>MQRLSPGEFKTLISKERKSHFITPFALVYKTFCDLGYDQKNSDYFLNNPSEYIIAMRKNCWKEFEPFEKEFTTRMLSYLIDEERIKDMSPYDAIRDFTMEYPTHIYDLALSNTQSRRSRAGKEFESILELLMMGAGIPVD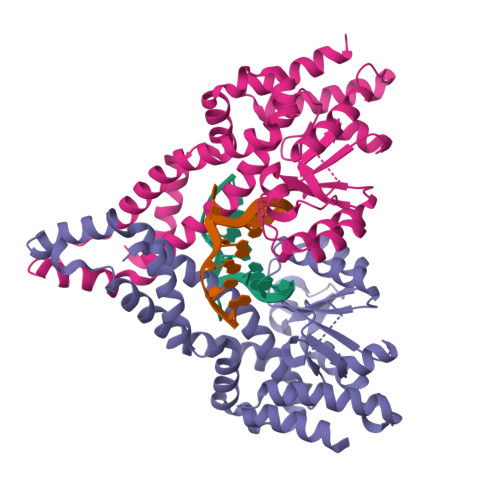VQGAIGKSFFQKNQIGKLVDLVMPGVVQYTSNKRNTMLISAKTTLRERWQEVPEEVNRTGIREMYLATLDDSFSEETINILYEANVVVVTTVENKNFKYKNNNRVLTFEDMLQSAMELSRKWNNVSYTDSEKEEIQQSILKQIEKYSDFPYVVNYYRNRLSALFD[4x]>[3x]MWITQEITPYLRKEYTIEAKLLDVRSEHNILEIFKSKDFGEIAMLNRQLLFKNFLHIESELLAHMGGCTKKELKEVLIVDGFDLELAHQLFKYDTHIDFVQADEKILDSFISFFPHFHEVKNNKNFTHAKQLLDLDIKKYDLIFCLQEPDIHRIDGLKRMLKEDGVFISVAKHPLL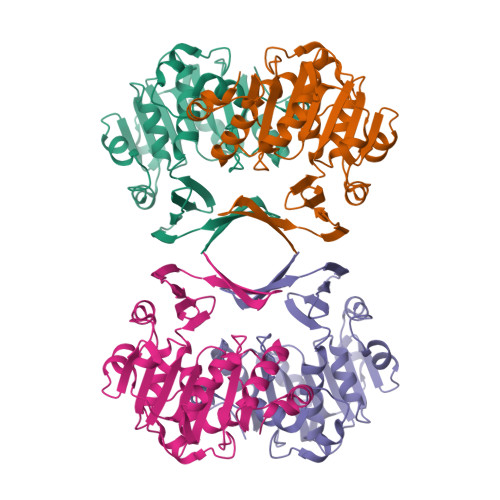EHVSMQNALKNMGGVFSVAMPFVAPLRILSNKGYIYASFKTHPLKDLMTPKIEALTSVRYYNEDIHRAAFALPKNLQEVFKDNIKS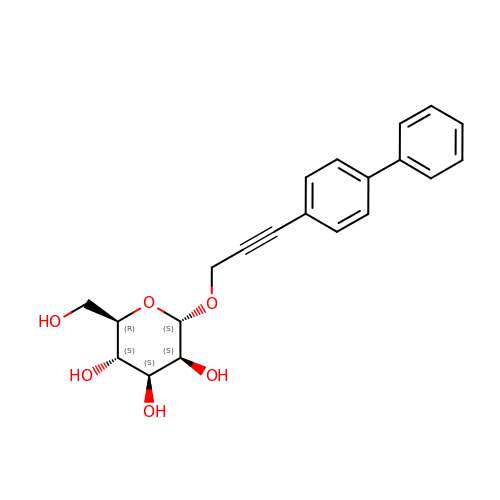(2R,3S,4S,5S,6S)-2-(hydroxymethyl)-6-[3-(4-phenylphenyl)prop-2-ynoxy]oxane-3,4,5-triol | C21 H22 O6 | UEPMXFZVTJIHES-MJCUULBUSA-N>[3x]MLAKRIIACLDVKDGRVVKGTNFENLRDSGDPVELGKFYSEIGIDELVFLDITASVEKRKTMLELVEKVAEQIDIPFTVGGGIHDFETASELILRGADKVSINTAAVENPSLITQIAQTFGSQAVVVAIDAKRVDGEFMVFTYSGKKNTGILLRDWVVEVEKRGAGEILLTSIDRDGTKSGYDTEMIRFVRPLTTLPIIASGGAGKMEHFLEAFLAG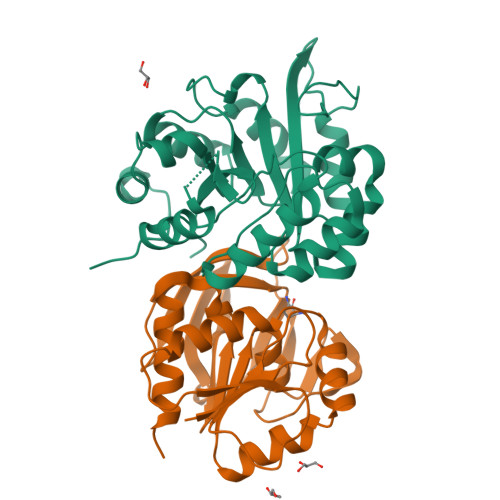ADAALAASVFHFREIDVRELKEYLKKHGVNVRLEGL;>[3x]MRIGIISVGPGNIMNLYRGVKRASENFEDVSIELVESPRNDLYDLLFIPGVGHFGEGMRRLRENDLIDFVRKHVEDERYVVGVCLGMQLLFEESEEAPGVKGLSLIEGNVVKLRSRRLPHMGWNEVIFKDTFPNGYYYFVHTYRAVCEEEHVLGTTEYDGEIFPSAVRKGRILGFQFHPEKSSKIGRKLLEKVIECSLSRR>MGSSHHHHHHSSGRENLYFQG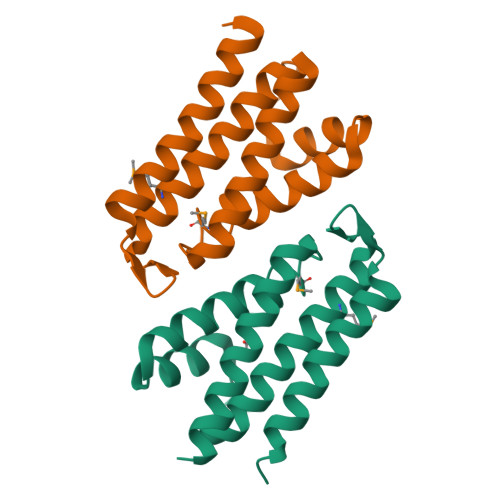HMIKKQELSAQEAVIEAKRYLNNAKDILRDKGGKEDGFYQDSKYVKMAGHTAYSGVLFALDHYFGKKTKGRKDVDWYKSNLAQQDKKILNTFVSVYEQLHLVMAYDGVGDAEVVKLGFQRAEIIIDWVERRLAAGS[4x]> SESQTLDKVYQMKSKPRGYCLIINNHNFAKAREKVPKLHSIRDRNGTHLDAGAL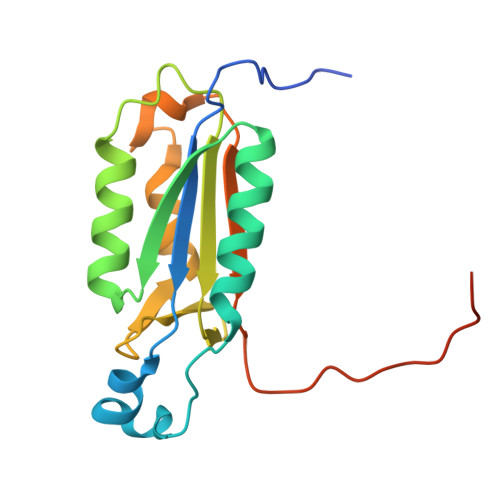TTTFEELHFEIKPHDDCTVEQIYEILKIYQLMDHSNMDCFICCILSHGDKGIIYGTDGQEAPIYELTSQFTGLKCPSLAGKPKVFFIQACQGDNYQKGIPVETDSEEQPYLEMD> MEHAVIVENVTKKYKLFKRTSERLLDMILPGGYGEDFYALRNVSFTADKGDVIGIVGVNGSGKSTLSNIIAGILPPTSGTIKIDGQASLIAISSGLNNQLT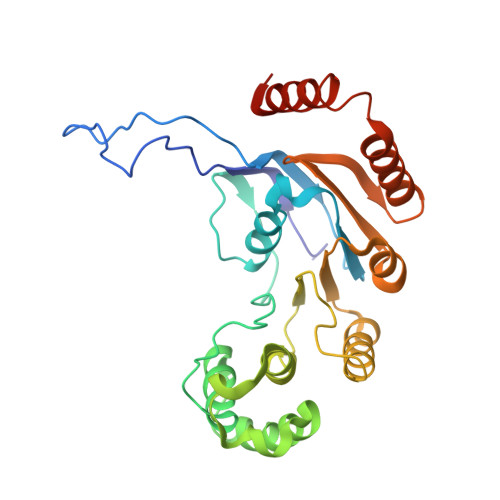GRENIELKCLMLGFSKKQIRAMEPDIIEFADIGKFIDQPVKTYSSGMKSRLGFAISVNIDPDVLVIDEALSVGDQTFADKCLDKMNEFKERGKTIFFISHSIGQVKSFCEKALWLEYGEVRGYGTVAEIIPQYEKFLKEYRAMSDKEKRQYKERVMRKQQGEFLQAAVK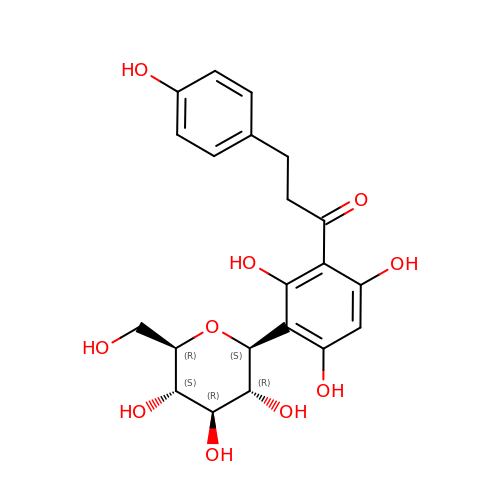1-[3-[(2S,3R,4R,5S,6R)-6-(hydroxymethyl)-3,4,5-tris(oxidanyl)oxan-2-yl]-2,4,6-tris(oxidanyl)phenyl]-3-(4-hydroxyphenyl)propan-1-one | C21 H24 O10 | VZBPTZZTCBNBOZ-VJXVFPJBSA-N Neonicotinoids are a major insecticide class, displaying high selectivity to insects over vertebrates and have been widely used in pest control. Neonicotinoids bind to the orthosteric sites (normally occupied by the neurotransmitter ACh) of nAChRs at α/non-α or α/α subunit interfaces formed by seven loops (A, B, C, D, E, F and G) in the long N-terminal, extracellular domain. Of particular importance are the basic residues in loops D and G, which contribute to the selective actions of neonicotinoids on insect nAChRs. In an attempt to clarify the divergent mechanism of dinotefuran's interactions with the An. gambiae nAChRs tested, we cocrystallized it with the Lymnaea stagnalis AChBP (Ls-AChBP), which is not a nAChR but has been widely used as a surrogate for LBD in nAChR interactions, since no insect nAChR has been crystallized to date.

In this experiment, we employed the Ls-AChBP Q55R mutant as it mimics insect nAChRs in possessing the basic residue in loop D. Dinotefuran bound to all five orthosteric sites of the protein as observed for imidacloprid, thiacloprid, clothianidin and the nitromethylene analogue of imidacloprid. Of the dinotefuran stereoisomers, only the S-isomer cocrystallized with the Ls-AChBP, in line with the finding that the S-isomer was more potent than the R-isomer in binding to the housefly (Musca domestica nAChRs). In the Q55R mutant of Ls-AChBP, the guanidine moiety of dinotefuran stacked with Tyr185 in loop C as in other neonicotinoids. The nitro group interacted electrostatically with the Arg55 in loop D and Lys34 in loop G, confirming that these basic residues in loop D and loop G generally play an important role in the selective insect nAChR−neonicotinoid interactions. The non-aromatic tetrahydrofuran ring is a unique structure of dinotefuran not seen in other neonicotinoids. The tetrahydrofuran ring oxygen formed a hydrogen bond via water with the indole ring NH of Trp143 in loop B and the main chain carbonyl of Met114 in loop E as in the cases of the pyridine/thiazole nitrogen in the other neonicotinoids. Nevertheless, the tetrahydrofuran ring hydrogens undergo CH-N electrostatic interactions, which are not seen in the crystal structures of the Q55R mutant of Ls-AChBP in complex with imidacloprid, thiacloprid and clothianidin. Also, the guanidine NH of dinotefuran did not form a hydrogen bond with the main chain carbonyl of Trp143, as was the case for clothianidin. As such, the structural information supports the unique experimental binding interactions of dinotefuran with the An. gambiae nAChRs, with the caveat that the AChBP is only a surrogate, albeit useful model of the nAChR LBD. The protein was cocrystallized with 1 mM dinotefuran in precipitant solution composed of 16.5–18.0% PEG4000 and 0.2 M sodium citrate (pH 5.4) at 20°C. X-ray diffraction data were obtained at SPring-8 BL26B1 beamline at 100 K using a CCD detector RAYONIX MX225HE.

>[4x]SLDRADILYNIRQTSRPDVIPTQRDRPVAVSVSLKFINILEVNEITNEVDVVFWQRTTWSDRTLAWNSSHSPDQVSVPISSLWVPDLAAYNAISKPEVLTPQLARVVSDGEVLYMPSIRQRFSCDVSGVDTESGATCRIKIGSWTHHSREISVDPTTENSDDSEYFSQYSRFEILDVTQKKNSVTYSCCPEAYEDVEVSLNFRKKGRSEI;> LDRADILYNIRQTSRPDVIPTQRDRPVAVSVSLKFINILEVNEITNEVDVVFWQRTTWSDRTLAWNSSHSPDQVSVPISSLWVPDLAAYNAISKPEVLTPQLARVVSDGEVLYMPSIRQRFSCDVSGVDTESGATCRIKIGSWTHHSREISVDPTTENSDDSEYFSQYSRFEILDVTQKKNSVTYSCCPEAYEDVEVSLNFRKKGR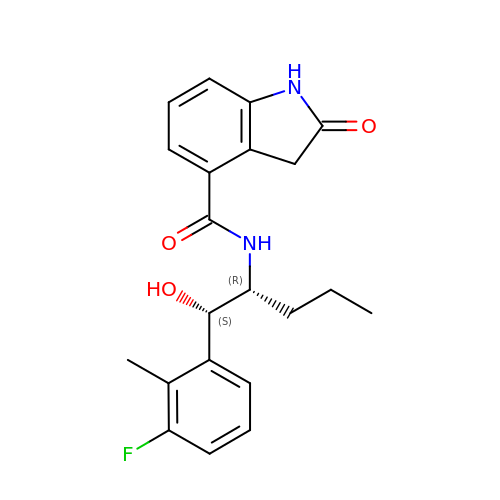~{N}-[(1~{S},2~{R})-1-(3-fluoranyl-2-methyl-phenyl)-1-oxidanyl-pentan-2-yl]-2-oxidanylidene-1,3-dihydroindole-4-carboxamide | C21 H23 F N2 O3 | MSZBLPYPBQYDNI-QUCCMNQESA-N> GSMKNLIAEANQAVEQFAGQVKARYYPAYHIAAKSGWINDPNGLIYFNNQYHVFFQHHPYNEQWGKIHWGHVVSDDLVHWRNLPIALAPSQEYDKDGCFSGCAIDDNGVLTLIYTGHVVLKEAGDKSVFKQVQCLATSKDGIHFEKQGVIVTPPEGIMHFRDPKVWRQDDQWYMVV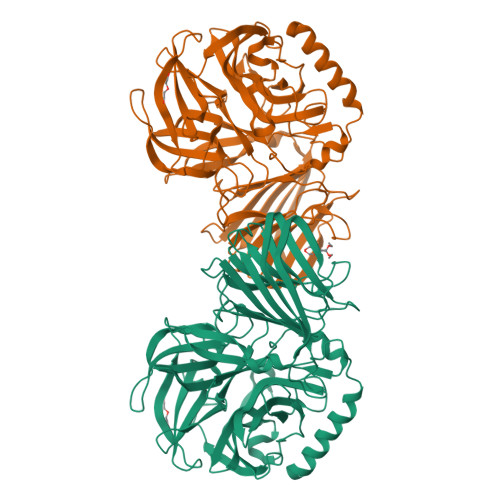GVNDHDNTGQVWLYHSQDLYHWQFVQVLAKMADPNVYMLECPDFFPLGDKYVLTCSPQGMKANGYHYRNRYQSGYIVGDWQPGSAFTITQDFTELDFGHDYYAPQTLISHDQRRIVIAWMDMWDSVMPSQADKWAGVLTLPRTLMLSSNNKLLINPITELKSLRGIQKKITSINLSNAIQDLQLDSMQCELILKIDLTNSDAERAGIALSASPDGKQSTLLYVDNQAQRVILDRTYSGEGMVGYRSVALPADKFLTLHIFIDHSSVEVFVNEGQATLTSRIYPTSEKRTLFLFAENGALRVEQLDYWQIKNMRG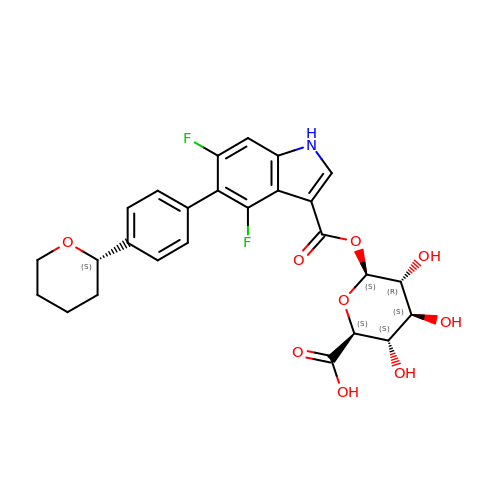1-O-(4,6-difluoro-5-{4-[(2S)-oxan-2-yl]phenyl}-1H-indole-3-carbonyl)-beta-D-glucopyranuronic acid | C26 H25 F2 N O9 | GZCJKJJWOUAGMR-WBTGXFMPSA-N>[2x]SNAMADEIAKAQVARPGGDTIFGKIIRKEIPAKIIFEDDRCLAFHDISPQAPT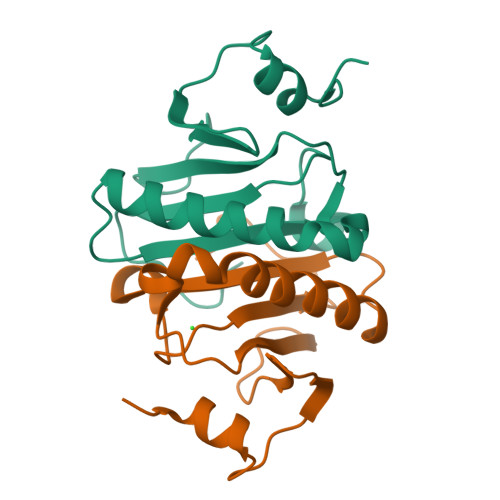HFLVIPKKHISQISVAEDDDESLLGHLMIVGKKRAADLGLNKGYRMVVNEGSDGGQSVYHVHLHVLGGRQMHWPPG The controller protein of the type II restriction–modification (RM) system Esp1396I binds to three distinct DNA operator sequences upstream of the methyltransferase and endonuclease genes in order to regulate their expression. The plasmid-borne type II RM system Esp1396I has been well studied both in vitro and in vivo and reveals a temporal control mechanism that employs a controller protein (C-protein) encoded within the RM operon. The controller protein C.Esp1396I, and indeed all other C-proteins studied to date, have been shown to be homodimeric helix–turn–helix proteins that bind to pseudo-symmetrical DNA operator sequences. Each of these two structures, termed 19OR and 25OL, are nucleoprotein complexes comprising a C-protein dimer and a DNA duplex.

The 19OR structure includes the entire OR C-protein binding site. The 19OR crystals showed weak isotropic diffraction extending to 3 Å resolution. The structure was refined in space group C2 with one copy of the complex per asymmetric unit. In the 19OR crystal structure, each protein dimer contacts four DNA duplexes and two protein subunits belonging to adjacent asymmetric units. The only clear contacts between the C-­protein and the DNA occur between the protein side chains and the phosphate groups in the DNA backbone. The overall conformation of the DNA duplex in the 19OR structure does not conform to the canonical B-form; it is significantly distorted and resembles the biologically bound conformation previously observed in the 19OL structure. The overall bend of 42° is a little less than that observed in the biologically bound OL complex (54°), but the DNA retains the reduced minor groove in the central spacer between the two C-boxes, despite the lack of significant interactions with the HTH motif. The bend in the DNA is centred at the TATA sequence between the C-boxes, as observed in other C-protein complexes. The 19OR structure presented here shows that even in the absence of specific protein–DNA contacts the DNA sequence at the OR operator is compressed at the minor groove, greatly reducing the energy penalty of DNA distortion following C-protein binding.

>[2x]GSHMESFLLSKVSFVIKKIRLEKGMTQEDLAYKSNLDRTYISGIERNSRNLTIKSLELIMKGLEVSDVVFFEMLIKEILKHD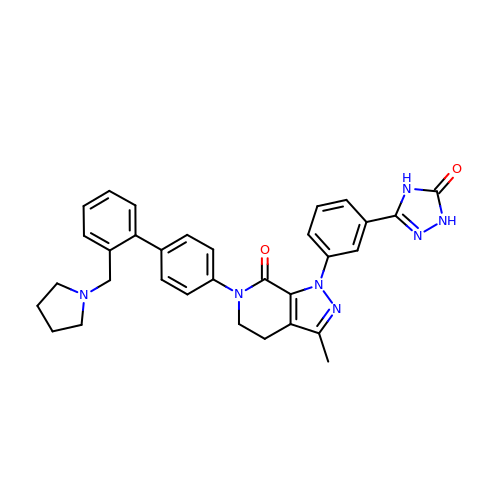3-METHYL-1-(3-(5-OXO-4,5-DIHYDRO-1H-1,2,4-TRIAZOL-3-YL)PHENYL)-6-(2'-(PYRROLIDIN-1-YLMETHYL)BIPHENYL-4-YL)-5,6-DIHYDRO-1H-PYRAZOLO[3,4-C]PYRIDIN-7(4H)-ONE | C32 H31 N7 O2 | DBOPERRYUICVTA-UHFFFAOYSA-N> MAAQGFLLIATFLLVLMVLARPLGSGLARLINDIPLPGTTGVERVLFRALGVSDREMNWKQYLCAILGLNMLGLAVLFFMLLGQHYLPLNPQQLPGLSWDLALNTAVSFVTNTNWQSYSGETTLSYFSQMAGLTVQNFLSAASGIAVIFALIRAFTRQSMSTLGNAWVDLLRITLWVLVPVALLIALFFIQQGALQNFLPYQAVNTVEGAQQLLPMGPVASQEAIKMLGTNGGGFFNANSSHPFENPTALTNFVQMLAIFLIPTALCFAFGEVMGDRRQGRMLLWAMSVIFVICVGVVMWAEVQGNPHLLALGTDSSINMEGKESRFGVLVSSLFAVVTTAASCGAVIAMHDSFTALGGMVPMWLMQIGEVVFGGVGSGLYGMMLFVLLAVFIAGLMIGRTPEYLGKKIDVREMKLTALAILVTPTLVLMGAALAMMTDAGRSAMLNPGPHGFSEVLYAVSSAANNNGSAFAGLSANSPFWNCLLAFCMFVGRFGVIIPVMAIAGSLVSKKSQAASSGTLPTHGPLFVGLLIGTVLLVGALTFIPALALGPVAEYLS;> MSRKQLALFEPTLVVQALKEAVKKLNPQAQWRNPVMFIVWIGSLLTTCISIAMASGAMPGNALFSAAISGWLWITVLFANFAEALAEGRSKAQANSLKGVKKTAFARKLREPKYGAAADKVPADQLRKGDIVLVEAGDIIPCDGEVIEGGASVDESAITGESAPVIRESGGDFASVTGGTRILSDWLVIECSVNPGETFLDRMIAMVEGAQRRKTPNEIALTILLIALTIVFLLATATLWPFSAWGGNAVSVTVLVALLVCLIPTTIGGLLSAIGVAGMSRMLGANVIATSGRAVEAAGDVDVLLLNKTGTITLGNRQASEFIPAQGVDEKTLADAAQLASLADETPEGRSIVILAKQRFNLRERDVQSLHATFVPFTAQSRMSGINIDNRMIRKGSVDAIRRHVEANGGHFPTDVDQKVDQVARQGATPLVVVEGSRVLGVIALKDIVKGGIKERFAQLRKMGIKTVMITGDNRLTAAAIAAEAGVDDFLAEATPEAKLALIRQYQAEGRLVAMTGDGTNDAPALAQADVAVAMNSGTQAAKEAGNMVDLDSNPTKLIEVVHIGKQMLMTRGSLTTFSIANDVAKYFAIIPAAFAATYPQLNALNIMCLHSPDSAILSAVIFNALIIVFLIPLALKGVSYKPLTASAMLRRNLWIYGLGGLLVPFIGIKVIDLLLTVCGLV;> MSGLRPALSTFIFLLLITGGVYPLLTTVLGQWWFPWQANGSLIREGDTVRGSALIGQNFTGNGYFHGRPSATAEMPYNPQASGGSNLAVSNPELDKLIAARVAALRAANPDASASVPVELVTASASGLDNNITPQAAAWQIPRVAKARNLSVEQLTQLIAKYSQQPLVKYIGQPVVNIVELNLALDKLDE;> MSAGVITGVLLVFLLLGYLVYALINAE

KdpFABC is a high-affinity prokaryotic K+ uptake system that forms a functional chimera between a channel-like subunit (KdpA) and a P-type ATPase (KdpB). The heterotetrametric KdpFABC complex comprises four subunits, namely the channel-like KdpA, a member of the superfamily of K+ transporters (SKT), the P-type ATPase KdpB, the lipid-like stabilizer KdpF, and KdpC, whose function is still unknown. At high K+ levels, KdpFABC needs to be inhibited to prevent excessive K+ accumulation to the point of toxicity. This is achieved by a phosphorylation of the serine residue in the TGES162 motif in the A domain of the pump subunit KdpB (KdpBS162-P).

To further investigate the role of the tight state in the conformational cycle of KdpFABC, we prepared a cryo-EM sample of KdpFABS162-P/D307NC under nucleotide-free conditions. This mutant is catalytically inactive and thus restricted to E1 states preceding phosphorylation in the P domain. We have termed this state the E1 apo open state, as the N and P domains are far apart to provide access to the nucleotide-binding site. The high degree of flexibility of the N domain in these open states could facilitate nucleotide binding at the start of the Post-Albers cycle. The second state, featuring one structure resolved globally at 3.4 Å and represented by 19% of the initial particle set, shows a compact conformation of the cytosolic domains with the N and A domains in close contact, providing no space for a nucleotide to bind. The presence of a similar tight conformation in both the E1P and the E1 apo states of KdpBS162-P shows that, while the inhibitory KdpBS162 phosphorylation appears to be a prerequisite, the observed close association of the N and A domains can occur before or after the binding and cleavage of ATP. EPR analysis of KdpFABS162-P/D307NC in the absence of nucleotide resulted in distances that resemble the E1 apo tight (34%) and the E1 apo open (66%) states. This corroborates the cryo-EM results that both tight and open states are adopted in the same sample at nucleotide-free conditions. Notably, the E1 apo tight state likely has no major physiological relevance, as in the presence of ATP, it would progress through the catalytic cycle up to the point of inhibition.> CCGATACCGG;> CCGGTATCG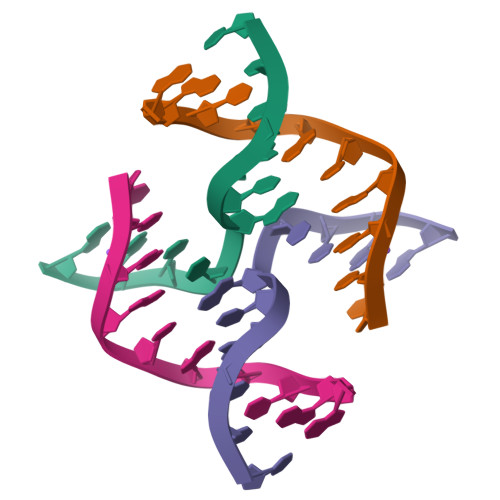G>[4x]SNARVFNFAAGPATLPENVLLKAQADLYNWRGSGMSVMEMSHRGKEFLSIIQKAESDLRQLLEIPQEYSVLFLQGGATTQFAALPLNLCKSDDTVDFVVTGSWGDKAVKEAKKYCKTNVIWSGKSEKYTKVPSFEELEQTPDAKYLHICANETIHGVEFKDYPVPKNGFLVADMSSNFCSKPVDVSKFGVIYGGAQKNVGPSGVTIVIIRKDLIGNAQDITPVMLDYKIHDENSSLYNT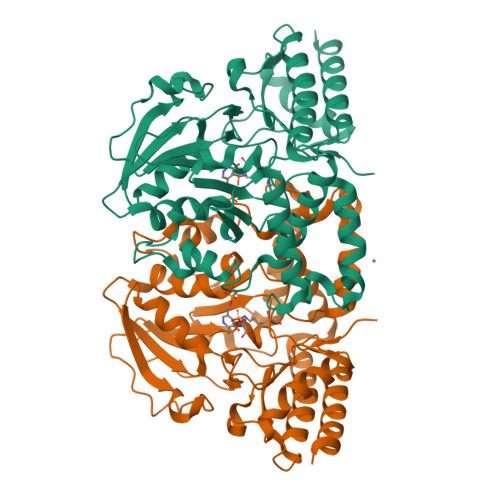PPCFGIYMCGLVFEDLLEQGGLKEVEKKNQRKADLLYNAIEESNGFFRCPVEKSVRSLMNVPFTLEKSELEAEFIKEAAKEKMVQLKGHRSVGGMRASIYNAMPLAGVEKLVAFMKDFQAKHA>[4x]GSHMAAGGDHGSPDSYRSPLASRYASPEMCFVFSDRYKFRTWRQLWLWLAEAEQTLGLPITDEQIREMKSNLENIDFKMAAEEEKRLRHDVMAHVHTFGHCCPKAAGIIHLGATSCYVGDNTDLIILRNALDLLLPKLARVISRLADFAKERASLPTLGFTHFQPAQLTTVGKRCCLWI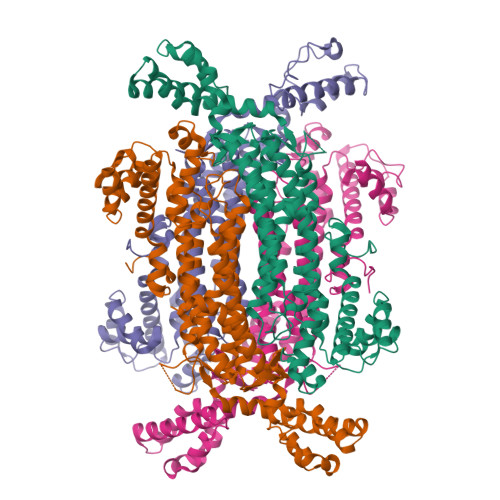QDLCMDLQNLKRVRDDLRFRGVKGTTGTQASFLQLFEGDDHKVEQLDKMVTEKAGFKRAFIITGQTYTRKVDIEVLSVLASLGASVHKICTDIRLLANLKEMEEPFEKQQIGSSAMPYKRNPMRSERCCSLARHLMTLVMDPLQTASVQWFERTLDDSANRRICLAEAFLTADTILNTLQNISEGLVVYPKVIERRIRQELPFMATENIIMAMVKAGGSRQDCHEKIRVLSQQAASVVKQEGGDNDLIERIQVDAYFSPIHSQLDHLLDPSSFTGRASQQVQRFLEEEVYPLLKPYESVMKVKAELCL>MSAQKRITLYMASASPFPHRVRLALEEAHATYEMIHISLVDKQDWYQKKVYPDRAQVPYLIYGGPELHPDEAPSPDAAKIPESLVILEFLADLFPAAHLLPSDPVLRARARLFTTAVETELLPAQKAFFLMGGPPDAMLAALDALQARLPPAGGFAAGPQWSIADAAVMPILLRLRMSVTLEVGFFAPGAAPVVRAALESPRFARLQRYIADNVARPSMAA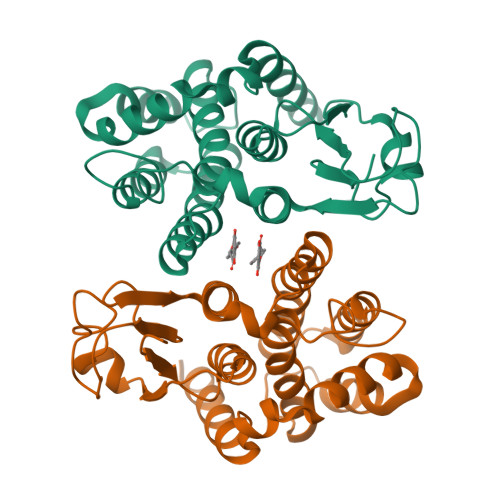TWDEAAVKAEFVGRFEKLRSLKAAQHHHHHH[4x]> MRGSHHHHHHGSAVSAKIEIYTWSTCPFCMRALALLKRKGVEFQEYCIDGDNEAREAMAARANGKRSLPQIFI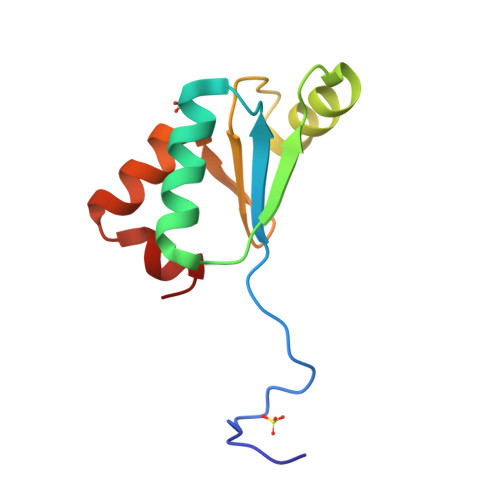DDQHIGGCDDIYALDGAGKLDPLLHS>[2x]MSNENKTIHDFELNLICDFFSNMERQGPGSPEVTLKA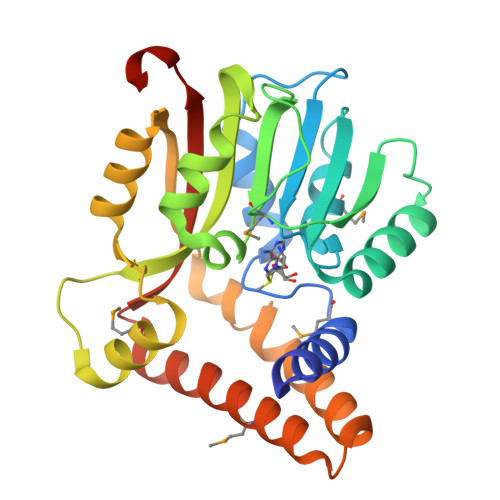LSFIDNLTEKSLIADIGCGTGGQTMVLAGHVTGQVTGLDFLSGFIDIFNRNARQSGLQNRVTGIVGSMDDLPFRNEELDLIWSEGAIYNIGFERGLNEWRKYLKKGGYLAVSECSWFTDERPAEINDFWMDAYPEIDTIPNQVAKIHKAGYLPVATFILPENCWTDHYFTPKVAAQKIFLTKYAGNKIAEEFSMLQSIEEELYHKYKEYYGYTFFIAKKIRLLEHHHHHH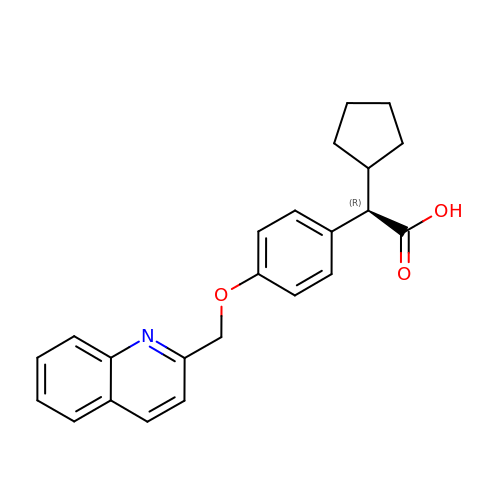(2R)-cyclopentyl{4-[(quinolin-2-yl)methoxy]phenyl}acetic acid | C23 H23 N O3 | ZEYYDOLCHFETHQ-JOCHJYFZSA-N> MSGQFTGTGTGGDVFKVDLNEQFDRADMVWIGTASVLVWIMIPGVGLLYSGISRKKHALSLMWAALMAACVAAFQWFWWGYSLVFAHNGSV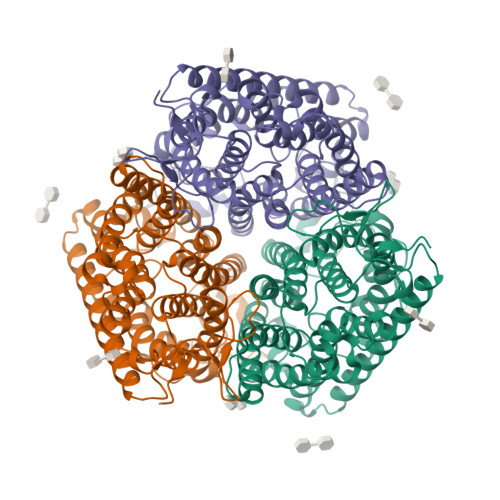FLGTLQNFCLKDVLGAPSIVKTVPDILFCLYQGMFAAVTAILMAGAGCERARLGPMMVFLFIWLTVVYCPIAYWTWGGNGWLVSLGALDFAGGGPVHENSGFAALAYSLWLGKRHDPVAKGKVPKYKPHSVSSIVMGTIFLWFGWYGFNGGSTGNSSMRSWYACVNTNLAAATGGLTWMLVDWFRTGGKWSTVGLCMGAIAGLVGITPAAGYVPVYTSVIFGIVPAIICNFAVDLKDLLQIDDGMDVWALHGVGGFVGNFMTGLFAADYVAMIDGTEIDGGWMNHHWKQLGYQLAGSCAVAAWSFTVTSIILLAMDRIPFLRIRLHEDEEMLGTDLAQIGEYAYYADDDPETNPYVLEPIRDTTISQPLPHIDGVADGSSNNDSGEAKNHHHHHH> MELIRIAMKKDLENDNSLMNKWATVAGLKNPNPLYDFLNHDGKTFNEFSSIVNIVKSQYPDREYELMKDYCLNLDVKTKAARSALEYADANMFFEIEDVLIDSMISCSNMKSKEYGKVYKIHRELSNSVITEFEAVKRLGKLNIKTPEMNSFSRLLLLYHYLSTGNFSPMAQLIKQIDLSEISENMYIRNTYQTRVHVLMSNIKLNENSLEECREYSKKALESTNILRFQVFSYLTIGNSLLFSNYELAQENFLKGLSISVQNENYNMIFQQALCFLNNVWRKENKWINFESDSIMDLQEQAHCFINFNENSKAKEVLDKLDLLVHNDNELAMHYYLKGRLEQNKACFYSSIEYFKKSNDKFLIRLPLLELQKMGENQKLLE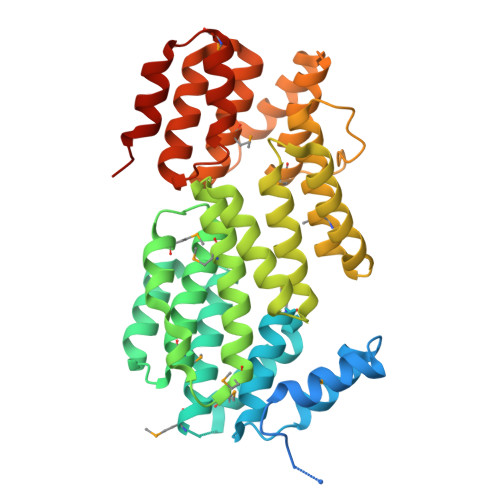LLLLLEHHHHHHHH Here, by solving the crystal structure, it is shown that MtGlu5 from Meiothermus taiwanensis WR-220, a GH5-family endo-β-1,4-glucanase (EC 3.2.1.4), has a bipartite architecture consisting of a Cel5A-like catalytic domain with a (β/α)8 TIM-barrel fold and an inserted CBM29-like noncatalytic domain with a β-jelly-roll fold. MtGlu5 contains a Cel5A-like CD similar to TmCel5A from Thermotoga maritima, but has an additional novel domain inserted into an internal site in the CD. Unlike other known cellulases with CBMs at the termini, this inserted CBM in the newly identified MtGlu5 acts in synergy with the CD, as demonstrated by ITC experiments.

Subsequently, sugar-bound crystals of wild-type MtGlu5 were obtained by substrate co-crystallization with carboxy­methyl cellulose (CMC). However, it turned out to contain only one protein molecule in the asymmetric unit, with a high solvent content of ∼70%. In the refined model of MtGlu5, the conserved CD has a (β/α)8 TIM-barrel fold and the inserted CBM shows a β-jelly-roll fold. Presumably, some CMC in the crystallization solution had been hydrolyzed by the active wild-type enzyme. In the catalytic pocket, the glucose molecule is sandwiched between the indole side chains of Trp43 and Trp224, which are presumably engaged in stacking interactions. The binding site is adjacent to the two conserved catalytic residues Glu149 and Glu393. It corresponds to the −2 or −3 sugar of a bound cellulose substrate, according to the general nomenclature. The other sugar units were not observed because they were considered to be leaving products and were not properly retained in the active site. Notably, the inserted CBM is not a fixed attachment, as its orientation varies with respect to the CD in the monoclinic and tetragonal crystals of iMtGlu5 and MtGlu5.

> MGCQSTQLQTPAPDTGGIVELNRQLGRGVNLGNALEAPWEGAWGVRLEEGFFELIREAGFKTIRLPVSWTHHAGRAAPYTIDPAFFSRVDWAVTQATRRGLNIVVNVHHYDELNANPQAEEARYLSIWRQIAERYRNQPGSVYFELLNEPHGRFNDNPQLWNDLLAKALRVVRESNPSRAVIVGPVGWNSLWRLSELRLPDDPNLIVTFHYYDPLEFTHQGAEWLNPVPPTGVVWRENQGAFAAGWQNWSWGSRVGFVGEALEITYQEGWAGFYLHSDAGVEGYDRLAFRTSAPVSLQVSCRRDAPAKAVTTSGGVETVVNLSECGNPSRLTDLILQNNSPNARAAFRLERLELRGPGSPLALLTHQQNAIAQAMEFAQRWAEQNRRPIFVGEFGAYEKGDLDSRVRWTGAVRSELEKRNFSWAYWEFAAGFGIYDRTTRQWRTPLLKALVPEQPKLAAALEHHHHHH>[2x]MMKRYLLTLAAFAALGALAQSPTLTIYSGRGQSLVEPLVKQFEAETGIRVQVRYSTDAQILAALQEEGSRSPADLFWANTAGALGQASAKGLLRPLGETLLEKPIAFVPASRTWVPVTVRLRVLAYNPDRIKAEELPESLLDLPRFAREKGLVGRVGWTPTYSSFQDMVAGMIALYGEEKTREWLLAMKALAPKAYPSNPAMLDAIRAGEVDLGSTNHYYVVRF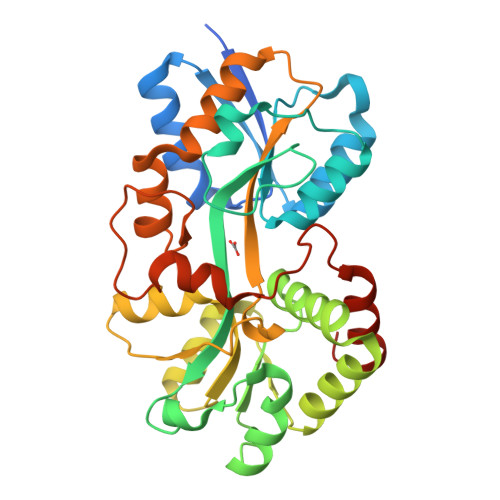RRAGYRLGMHHFRDGDAGNLALVTGAGLLKTSKNLAAATRFLTYLLSPQAQQYFVGNIGEYPLVKGVALDPNLLPLEEALAKSPKLDLEKLPLDRALRLLRETGVLHHHHHH> GSHMASLKDLEGKWRLMESHGFEEYMKELGVGLALRKMAAMAKPDCIITCDGNNITVKTESTVKTTVFSCNLGEKFEETTADGRKTETVCTFQDGAL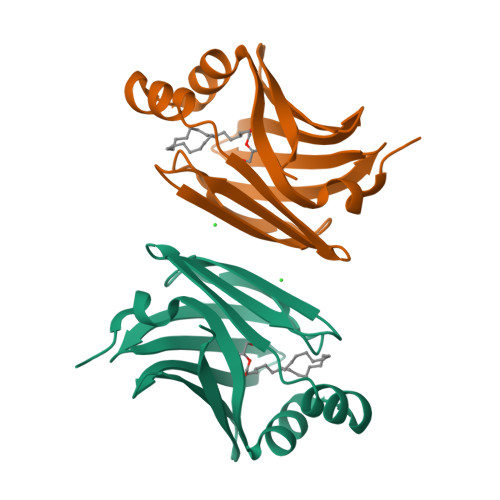VQHQQWDGKESTITRKLKDGKMIVECVMNNATCTRVYEKVQ> MPGDHRRIRGPEESQ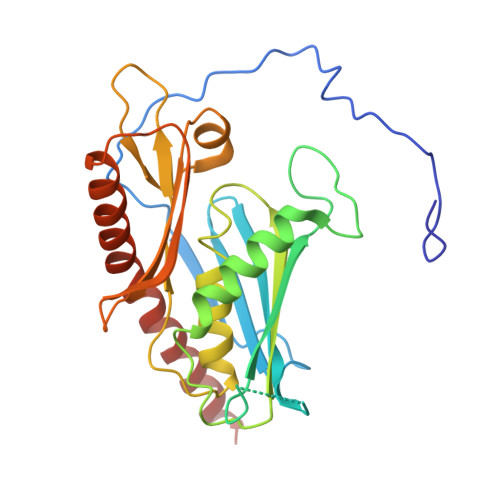PPQLYAADEEEAPGTRDPTRLRPVYARAGLLSQAKGSAYLEAGGTKVLCAVSGPRQAEGGERGGGPAGAGGEAPAALRGRLLCDFRRAPFAGRRRRAPPGGCEERELALALQEALEPAVRLGRYPRAQLEVSALLLEDGGSALAAALTAAALALADAGVEMYDLVVGCGLSLAPGPAPTWLLDPTRLEEERAAAGLTVALMPVLNQVAGLLGSGEGGLTESWAEAVRLGLEGCQRLYPVLQQSLVRAARRRGAAAQP>[6x]MAEQAVPYGRKTQHTPALKEVHILWITAGLGCDGDSVSITAASQPSVEDVVLGAIPGLPKVHLHNPVLAYENGDEFMAPFHKAARGEIDNFVLVLEGSIPNERINGEGYWAAMGTDPQTHQPITIPEWLDRLAPKALAVVGAGTCATYGGIHAMEGNPTGCMGLADYLGWQWKSRAGLPIVNVPGCP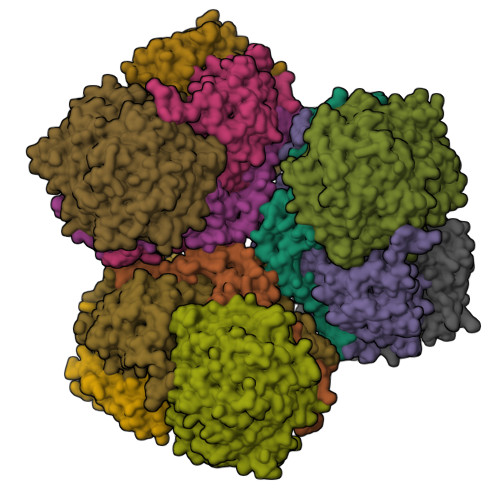VQPDNFMETLLYLLYQLAGLAPMIPLDEALRPKWLFTRTVHDGCDRAGSYEQAIFATEYGNPNCIVKLGCWGPVVQCNVPKRGWIAGVGGCPNVGGICIGCTMPGFPDKFMPFMDAPPGAVLSSNLIKSYGPLIRSLRKLTKDTLNDEPKWRHNQPVLTTGYRG;>[6x]MATIAAPGARPRAQAAPGKLVEMNWDPITRIVGSLGIYTKIDFENRRVAECYSTSSIFRGYSIFMKGKDPRDSHFITSRICGICGDNHATCSVYAQNMAYGVKPPPIADWIINLGEAAEYMFDHNIFQDNLVGVDFCEQMVRETNPGVWEKAKTAEAPHAAEHGYRTIADIMTALNPFTGEFYRETLLVSRYTREMFCLMEGRHVHPSTLYPGGVGTVPTIQLFTDYITRLMKYVEFMKKVVPLHDDLFDFFYEALPGYEEVGRRRILLGCWGSFQDPNVCDYNYRTMTKWGRGMFVTPGVVVDGELLTTDLVDINLNIRILLGSSFYQDWDHEETSVKNDPLGNAVDRKHPWNQTTLPRPQKRNFGGNYTWVMSPRWLDKRTGDHLALDTGGGPIARLWATALAGLVDIGYIKSTGHSVKIYLPRTALKPEAEFEWKIPMWSNAIERDRARTYFQAYSAAAALYFAEQALAELHAGRTRTFTDFKVPDEAIGCGFHEAVRGVLSHHLVIRDGKIANYHPYPPTPWNASPRDIYGTPGPYEDAVQNTPIFEENGPEKFKGIDIMRAVRSFDPCLPCGVH Aldehyde dehydrogenase 1A3 (ALDH1A3) belongs to an enzymatic superfamily composed by 19 different isoforms, with a scavenger role, involved in the oxidation of a plethora of aldehydes to the respective carboxylic acids, through a NAD+-dependent reaction. In particular, the ALDH1A subfamily is composed by three different isoforms (ALDH1A1, ALDH1A2 and ALDH1A3) which are involved in the conversion of retinal, an important mediator of vision, to the retinoic acid, a potent tissue differentiation factor for cellular development. Previous clinical studies highlighted the high expression of ALDH1A3 in cancer stem cells (CSCs) correlated to a higher risk of cancer relapses, chemoresistance and a poor clinical outcome.

NR6, showing the best inhibitory activity at 25 μM, was investigated further to determine its IC50 (5.3 ± 1.5 μM) and Ki (3.7 ± 0.4 μM) values, which revealed a potent and competitive model of inhibition. As detailed in the experimental procedures, we co-crystallized ALDH1A3 and NR6 and solved the complex structure at a final resolution of 2.9 Å. The final model contains two identical chains per asymmetric unit, arranged as dimer and a total of 38 solvent molecules. Our crystallographic data revealed that, in all monomers, NR6 binds to the enzyme at the entrance of the catalytic tunnel, and no direct interactions between the catalytic cysteine and the ligand are present. The NR6 heterocyclic cores lie in a conserved hydrophobic pocket located at the entrance of the catalytic tunnel. In this conformation, the phenyl ring in position 6 of the nucleus establishes contacts with the protein backbone, with Van der Waals contacts and hydrophobic interactions with the residues G136, R139, W189, N469, A470, L471 and Y472. Indeed, the cyanide group blocks the inhibitor in a rigid and conserved pose in both the monomers. As clearly shown in Figure 3C, the Y472 strongly binds and coordinates the pyridinic ring of NR6 with an edge-to-face π-π stacking interaction. All these interactions are further stabilized by a hydrogen bond that is established between the -OH group of the Y472 and the N1 of NR6 (3.7 Å). It is important to highlight that Y472 residue is not conserved in the ALDH1A1 and in the ALDH1A2, where it is substituted with a S461 and N478, respectively. Actually, the presence of the cyanide group promotes the distinct orientation of NR6 respect to Y472, thus stabilizing the binding with the protein and determining high selectivity towards ALDH1A3.

>MATANGAVENGQPDRKPPALPRPIRNLEVKFTKIFINNEWHESKSGKKFATCNPSTREQICEVEEGDKPDVDKAVEAAQVAFQRGSPWRRLDALSRGRLLHQLADLVERDRATLAALETMDTGKPFLHAFFIDLEGCIRTLRYFAGWADKIQGKTIPTDDNVVCFTRHEPIGVCGAITPWNFPLLMLVWKLAPALCCGNTMVLKPAEQTPLTALYLGSLIKEAGFPPGVVNIVPGFGPTVGAAISSHPQINKIAFTGSTEVGKLVKEAASRSNLKRVTLELGGKNPCIVCADADLDLAVECAHQGVFFNQGQCCTAASRVFVEEQVYSEFVRRSVEYAKKRPVGDPFDVKTEQGPQIDQKQFDKILELIESGKKEGAKLECGGSAMEDKGLFIKPTVFSEVTDNMRIAKEEIFGPVQPILKFKSIEEVIKRANSTDYGLTAAVFTKNLDKALKLASALESGTVWINCYNALYAQAPFGGFKMSGNGRELGEYALAEYTEVKTVTIKLGDKNP[2x]> MDIFREIASSMKGENVFISPPSISSVLTILYYGANGSTAEQLSKYVEKEADKNKDDISFKSMNKVYGRYSAVFKDSFLRKIGDNFQTVDFTDSRTVDAINKSVDIFTEGKINPLLDEPLSPDTSLLAISAVYFKAKWLMPFEKEFTSDYPFYVSPTEMVDVSMMSMYGEAFNHASVKESFGNFSIIELPYVGDTSMVVILPDNIDGLESIEQNLTDTNFKKWSDSMDAMFIDVHIPKFKVTGSYNLVDALVKLGLTE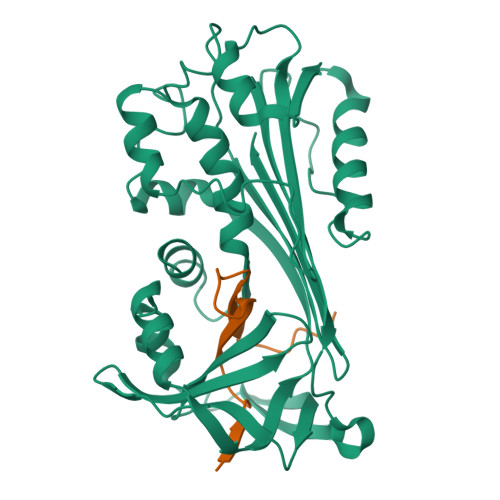VFGSTGDYSNMSNSDVSVDAMIHKTYIDVNEEYTEAAAATSAL;> VADSASTVTNEFSADHPFIYVIRHVDGKILFVGRYSSPTTN> MSKKPVALIILDGFALRDETYGNAVAQANKPNFDRYWNEYPHTTLKACGEAVGLPEGQMGNAEVGHLNIGAGRIVYQSLTRINIAIREGEFDRNETFLAAMNHVKQHGTSLHLFG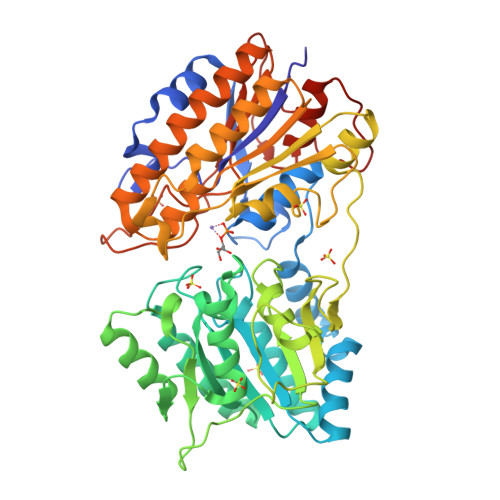LLSDGGVHSHIHHLYALLRLAAKEGVKRVYIHGFLDGRDVGPQTAPQYIKELQEKIKEYGVGEIATLSGRYYSMDRDKRWDRVEKAYRAMVYGEGPTYRDPLECIEDSYKHGIYDEFVLPSVIVREDGRPVATIQDNDAIIFYNFRPDRAIQISNTFTNEDFREFDRGPKHPKHLFFVCLTHFSETVAGYVAFKPTNLDNTIGEVLSQHGLRQLRIAETEKYPHVTFFMSGGREEEFPGEDRILINSPKVPTYDLKPEMSAYEVTDALLKEIEADKYDAIILNYANPDMVGHSGKLEPTIKAVEAVDECLGKVVDAILAKGGIAIITADHGNADEVLTPDGKPQTAHTTNPVPVIVTKKGIKLRDGGILGDLAPTMLDLLGLPQPKEMTGKSLIVK> MSDKLPYKVADIGLAAWGRKALDIAENEMPGLMRMRERYSASKPLKGARIAGCLHMTVETAVLIETLVTLGAEVQWSSCNIFSTQDHAAAAIAKAGIPVYAWKGETDEEYLWCIEQTLYFKDGPLNMILDDGGDLTNLIHTKYPQLLPGIRGISEETTTGVHNLYKMMANGILKVPAINVNDSVTKSKFDNLYGCRESLIDGIKRATDVMIAGKVAVVAGYGDVGKGCAQALRGFGARVIITEIDPINALQAAMEGYEVTTM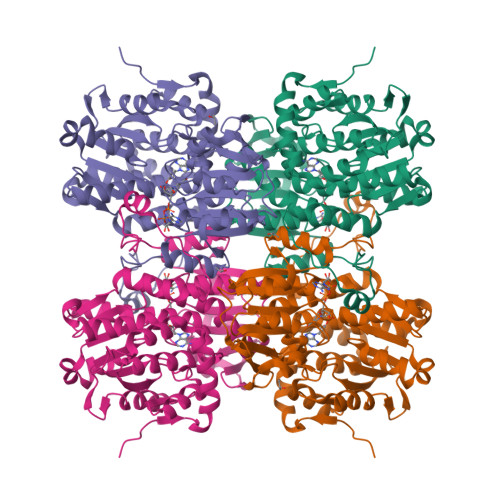DEACQEGNIFVTTTGCIDIILGRHFEQMKDDAIVCNIGHFDVEIDVKWLNENAVEKVNIKPQVDRYRLKNGRRIILLAEGRLVNLGCAMGHPSFVMSNSFTNQVMAQIELWTHPDKYPVGVHFLPKKLDEAVAEAHLGKLNVKLTKLTEKQAQYLGMSCDGPFKPDHYRY> PNYTKVEFGEHYARLRPKKLKANIEYTTPTGHIYRTDHKGRIKEVYVDNLSLKDGDRNSHAQRTVGGEDRLPDDDGGHLIARMFGGSKDIDNLVAQSKFINRPFKEKGHWYNLEKEWQEFLNSGKEVKNI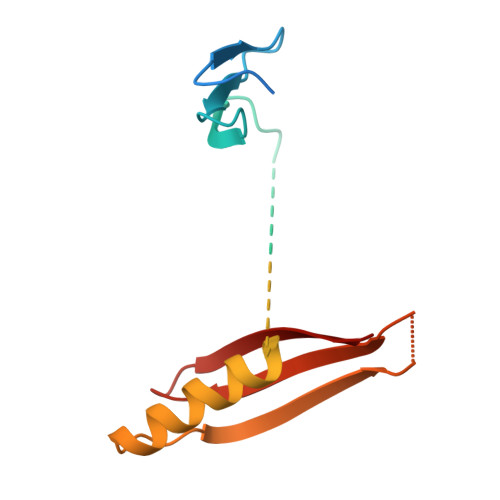KMEVKYSGNSQRPTIFKVEYEINGERNIRRILNK> HHHHHHVGVERT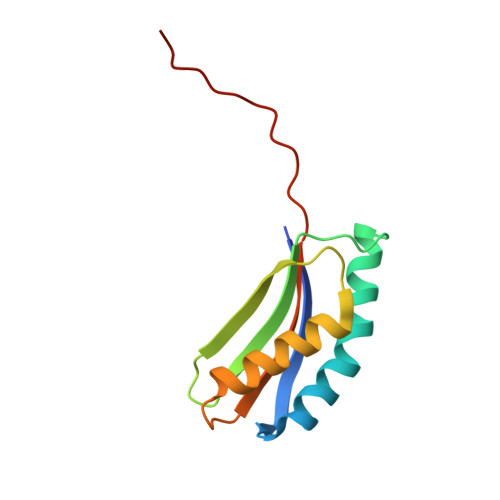MAEDIHHWSECEAIIERLYPELERRLAKVKPDLLIARQGVKLKFDDFQQTTQEHVWPRLNKADLIATARKTWDERRGGRGVRLVGLHVTLLDPQMERQLVLGL> MIVVKVGGAEGINYEAVAKDAASLWKEGVKLLLVHGGSAETNKVAEALGHPPRFLTHPGGQVSRLTDRKTLEIFEMVYCGLVNKRLVELLQKEGANAIGLSGLDGRLFVGRRKTAVKYVENGKVKVHRGDYTGTVEEVNKALLDLLLQAGYLPVLTPPALSYENEAINTDGDQIAALLATLYGAEALVYLSNVPGLLARYPDEASLVREIPVERIEDPEYLALAQGRMKRKVMGAVEAVRGGVKRVVFADARVENPIRRAL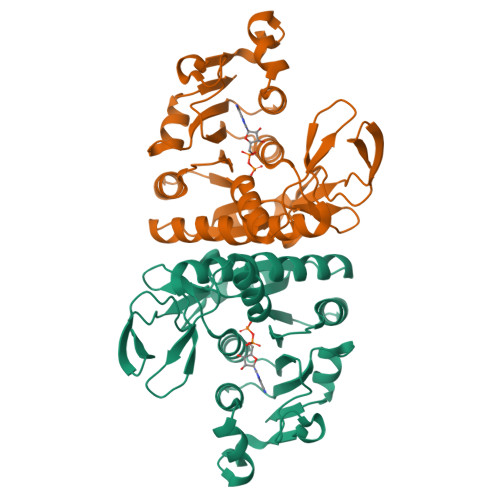SGEGTVVR>MASMGSSCSRSHSLSEAETTKNAKSADIDRRILQETKAEQHIHKLLLLGAGESGKSTIFKQIKLLFQTGFDEAELRSYTSVIHANVYQTIKILYEGAKELSQVESDSSKYVISPDNQEIGEKLSDIDGRLDYPLLNKELVLDVKRLWQDPAIQETYLRGSILQLPDCAQYFMENLVRLAEAGYVPTKEDVLYARVRTNGVVQIQFSPVGENKRGGEVYRLYDVGGQRNERRKWIHLFEGVNAVIFCAAISEYDQMLFEDETKNRMMETKELFDWVLKQRCFEKTSFILFLNKFDICEKKIQKVPLSVCEWFKDYQPIAPGKQEVEHAYEFVKKKFEELYFQSSKPDRVDRVFKIYRTTALDQKLVKKTFKLIDESMRRSREGT[4x]

In all organisms, the core G-protein complex consists of one subunit each of the α, β, and γ proteins and exists in bimodal active versus inactive states. Signaling is initiated when the bound GDP is exchanged for GTP on Gα, which results in conformational changes that dissociate the heterotrimeric complex into Gα·GTP and Gβγ. To avoid response saturation by active Gα proteins, faster deactivation is achieved with the help of GTPase activity accelerating proteins (GAP), such as the regulator of G-protein signaling (RGS), which binds to activated Gα to accelerate GTP-hydrolysis. The two domains of the Gα—the Ras-like domain and the helical domain (HD)—flank the guanine nucleotide binding site.

The x-ray crystal structures of the SmGPA·GTPγS and OsRGA1·GDP complexes were solved at 2.57 Å and 2.99 Å resolution, respectively, by molecular replacement using AtGPA1 as the search model. SmGPA crystallized with two monomers in the asymmetric unit and OsRGA1 crystallized with four monomers in the asymmetric unit. In comparison, the OsRGA1·GDP complex structure highlights how changes in the active site following GTP hydrolysis result in large-scale conformational change. Within the active site of the OsRGA1·GDP complex, interactions with the guanine ring and ribose of GDP are comparable to GTPγS bound in SmGPA, even with substitution of Tyr189 in OsRGA1 for the corresponding His186 of SmGPA. Although the backbone of the P-loop maintains position, multiple side chains from P-loop residues, such as Glu49, Ser50, and Lys52 in OsRGA1, shift. For switch I, the loss of the terminal phosphate breaks the key binding and catalytic interactions. In the OsRGA1·GDP structure, Thr194 (Thr191 in SmGPA) lacks an interaction partner and the catalytically critical Arg191 guanidino side-chain (Arg188 in SmGPA) points away from the active site. The loss of interactions with the bound ligand shifts the position of the β1b-α7 loop in switch I, which includes Arg191 and Thr194, away from the GTPase domain. Of the four OsRGA1 molecules in the asymmetric unit, three lacked electron density for residues corresponding to α8. Finally, the interaction between residues in switch III and the helical domain is broken, as the latter shifts away from the GTPase domain.>LPSDATPVLDVTGKELDPRLSYRIISTFWGALGGDVYLGKSPNSDAPCANGVFRYNSDVGPSGTPVRFIGSSSHFGQGIFEDELLNIQFAISTSKMCVSYTIWKVGDYDASLGTMLLETGGTIGQADSSWFKIVKSSQFGYNLLYCPVTTSSDDQFCLKVGVVHQNGKRRLA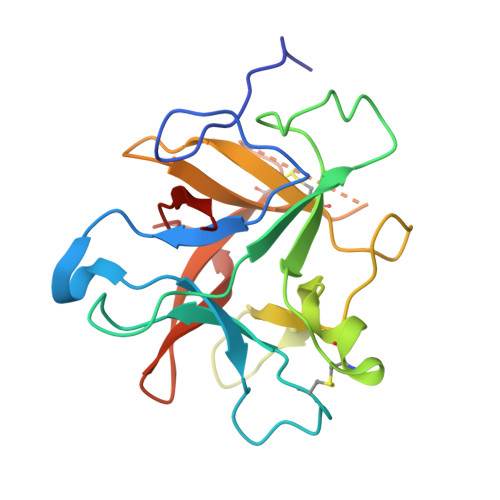LVKDNPLDVSFKQVQ[3x]>[2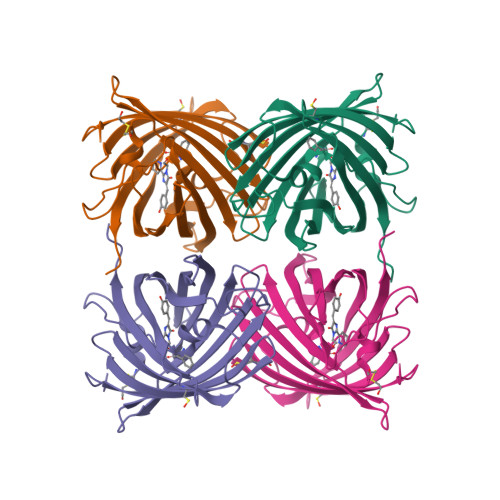x]MAHSKHGLKEEMTMKYHMEGCVNGHKFVITGEGIGYPFKGKQTINLCVIEGGPLPFSEDILSAGFKYGDRIFTEYPQDIVDYFKNSCPAGYTWGRSFLFEDGAVCICNVDITVSVKENCIYHKSIFNGMNFPADGPVMKKMTTNWEASCEKIMPVPKQGILKGDVSMYLLLKDGGRYRCQFDTVYKAKSVPSKMPEWHFIQHKLLREDRSDAKNQKWQLTEHAIAFPSALA>MSQHMIEQNYAEQSEFTLKAIGRNINYVLKEANHFSESSMLREDIQQTLSINHEVDQVVLAEYNRLLQRTFLFYTPSYSVHLYNFTGQLYNQGKIGYERFTYESLYKSPQVSEVIKLNGKPLWLGPYEFTESSANPNLFTSIRMINNTYTMNNMGILLQQFQFNNELNEIFNYFGTTHSKAVRFMLVNQEGLIMMDNKGKLSGRKLSDYAGSPVVLGAEYQSRKMTFDQVESVVSVHHLALDDFGKMNWNVVSVTPW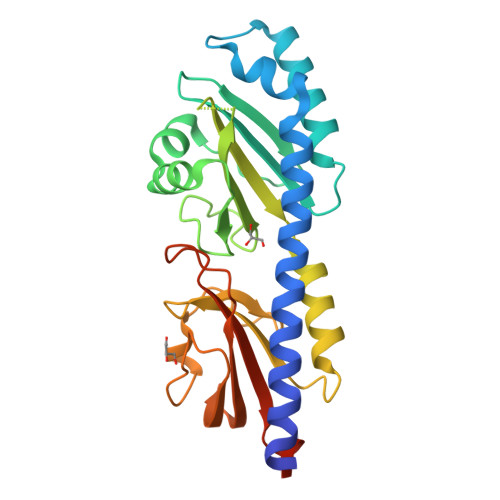EYLSGRSEQLEHHHHHH[2x]5-chloranyl-1,3-dihydroindol-2-one | C8 H6 Cl N O | 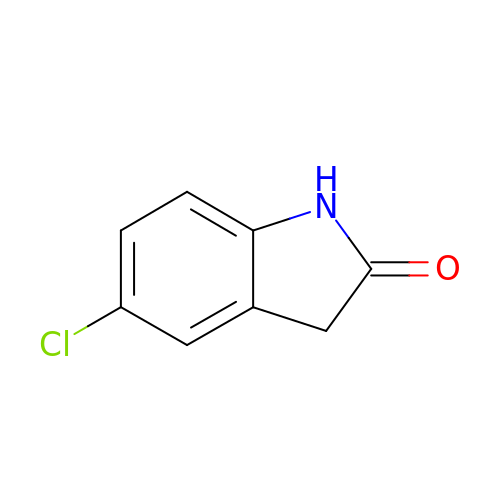WWJLCYHYLZZXBE-UHFFFAOYSA-N[4-({(3R)-1-[(1H-indol-3-yl)methyl]pyrrolidin-3-yl}amino)-2-nitrophenyl]methanol 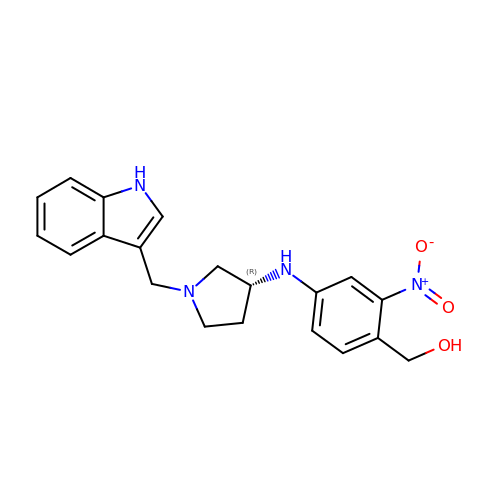| C20 H22 N4 O3 | LQBYYBOHEOEPPN-QGZVFWFLSA-N>MSLSASLPLAIERRPAAWT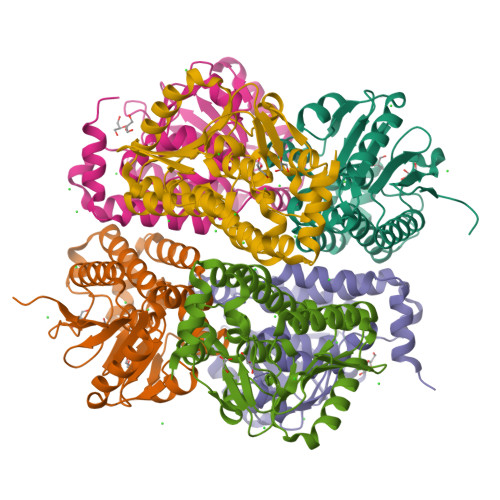FTLSRPEKRNALSAELVEALIDGVDAAHREQVPLLVFAGAGRNFSAGFDFTDYETQSEGDLLLRMVRIEMLLQRVAGSPSLTLALAHGRNFGAGVDLFAACKWRYCTPEAGFRMPGLKFGLVLGTRRFRDIVGADQALSILGSARAFDADEARRIGFVRDCAAQAQWPALIDAAAEAATALDPATRATLHRVLRDDHDDADLAALARSAAQPGFKARIRDYLAQPAAEGHHHHHH[6x]~{N}-[(3~{R},5~{S})-5-(hydroxymethyl)-1-methyl-pyrrolidin-3-yl]-2-(3-oxidanylidene-4~{H}-1,4-benzoxazin-6-yl)ethanamide 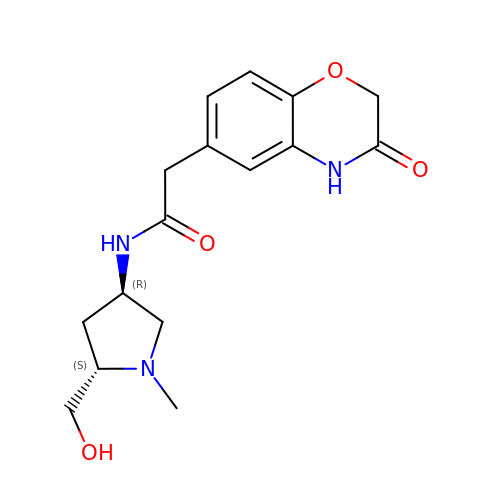| C16 H21 N3 O4 | GLBAXWCHBKFKRM-NEPJUHHUSA-N>AGGPGSRARAAGARGCRLRSQLVPVRALGLGHRSDELVRFRFCSGSCRRARSPHDLSLASLLGAGALRPPPGSRPVSQPCCRPTRYEAVSFMDVNSTWRTVD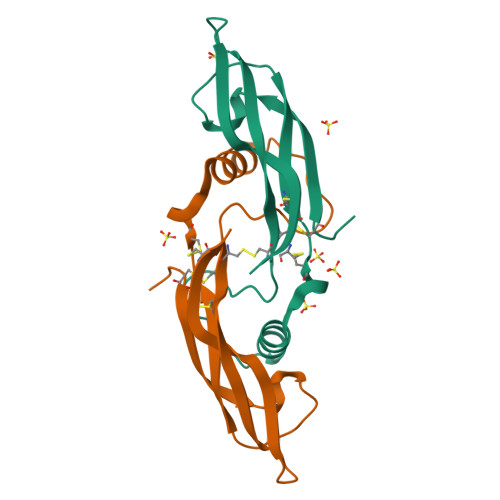RLSATACGCLG[2x]> MSKDYRSLANLSPFELKDELIKVASGKANRLMLNAGRGNPNFLATTPRRAFFRLGLFAAAESELSYSYMTVGVGGLAKLDGIEGRFERFIAE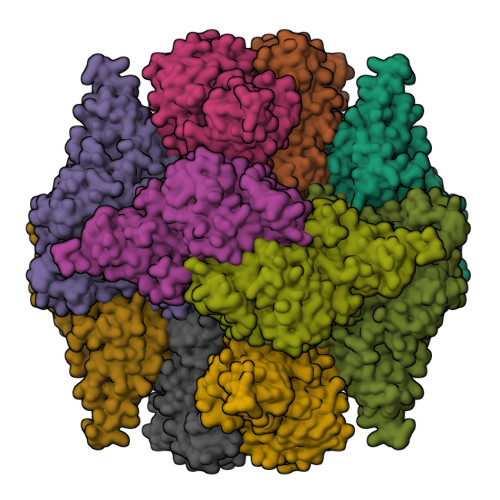HRDQEGVKFLGKSLSYVRDQLGLDPAAFLHEMVDGILGCNYPVPPRMLTVSEQIVRQYIVREMAGGAVPPESVDLFAVEGGTAAMAYIFESLRISGLLKAGDKVAIGMPVFTPYIEIPELAQYDLKEVPIHADPDNGWQYSDAELDKLKDPDVKIFFCVNPSNPPSVKMDQRSLDRVRAIVAEQRPDLLILTDDVYGTFADEFQSLFSVCPRNTLLVYSFSKYFGATGWRLGVIAAHKDNVFDHALSQLPESAKKALDHRYRSLLPDVRSLKFIDRLVADSRVVALNHTAGLSTPQQVQMVLFSLFALMDEADAYKQALKQLIRRREATLYRELGMPPLENPNSVNYYTLIDLQNVTCRLYGEAFSQWAVQQSSTGDMLFRVADETGIVLLPGRGFGSDRPSGRASLANLNEYEYAAIGRALRRLADELYEQYKALGKEKLAAALEHHHHHH>MGSSHHHHHHGSNAWEVNFDGLVGLTHHYAGLSFGNEASTRHRFQVSNPRLAAKQGLLKMKALADAGFPQAVIPPHERPFIPVLRQLGFSGSDEQVLEKVARQAPHWLSSVSSASPMWVANAATIAPSADTLDGKVHLTVANLNNKFHRSLEAPVTESLLKAIFNDEEKFSVHSALPQVALLGDEGAANHNRLGGHYGEPGMQLFVYGREEGNDTRPSRYPARQTREASEAVARLNQVNPQQVIFAQQNPDVIDQGVFHNDVIAVSNRQVLFCHQQAFARQSQLLANLRARVNGFMAIEVPATQVSVSDTVSTYL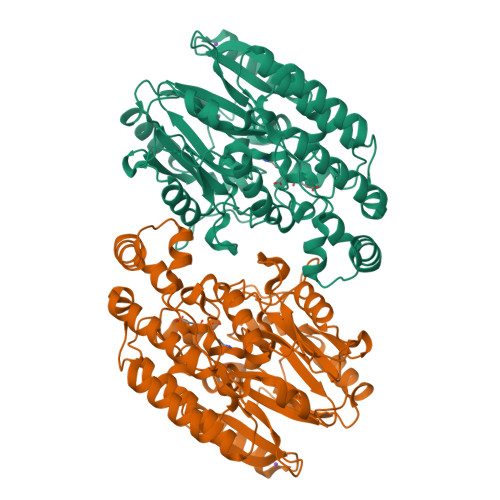FNSQLLSRDDGSMMLVLPQECREHAGVWGYLNELLAADNPISELKVFDLRESMANGGGPASLRLRVVLTEEERRAVNPAVMMNDTLFNALNDWVDRYYRDRLTAADLADPQLLREGREALDVLSQLLNLGSVYPFQREGGGNG[4x]Extensive experimental evidence has since demonstrated that cell division cycle protein 45 (Cdc45) is required throughout the process of DNA replication: it is essential for establishment of an initiation complex at DNA origins, and for chromosome unwinding and DNA synthesis at replication forks. More recently, Cdc45 was shown to be an integral component of the Cdc45-MCM-GINS (CMG) assembly responsible for DNA unwinding in the replisome. Recruitment of Cdc45 to the MCM2-7 heterohexamer is a key step in the highly regulated process that leads to the activation of helicase activity. Evidence concerning structure and function of Cdc45 remained elusive, until recent reports identified it as a remote orthologue of bacterial RecJ333435, a 5′-to-3′ single-stranded (ss) DNA exonuclease with multiple roles in DNA repair and a member of the DHH phosphoesterase superfamily.

The X-ray crystal structure of human Cdc45 was solved at 2.1 Å using the anomalous signal of crystals derivatized with the mercury compound thimerosal. A construct with an 11-residue excision (lacking amino acids S154 to I164) crystallized readily and was used for high-resolution structure determination. Crystallographic analysis reveals that human Cdc45 adopts a compact, disk-like shape, resulting from folding of the polypeptide chain into a closed arc, from its N- to the C-terminus. The only deviation from a globular fold is represented by a large helical insertion in the DHH domain, spanning amino acids L118 to S197, which projects away from the folded core of Cdc45 (discussed in detail later); the insertion consists of the low complexity, acidic region, which is almost entirely disordered, followed by the seven-turn helix α6 pointing away from the Cdc45 fold. Our crystallographic analysis shows that Cdc45 bears a remarkable three-dimensional similarity to the RecJ exonuclease, which reveals their homology despite very little sequence identity. The fold consists of an N-terminal DHH domain connected by a three-helix motif (α15 to α17) to a C-terminal DHH-Associated 1 (DHHA1) domain. Superposition with RecJ confirms the identification of Cdc45 residues that occupy equivalent positions to active-site residues in motifs I–IV of RecJ; the structure shows that three out of the four active-site motifs of Cdc45 contain inactivating mutations, providing a structural basis for its known lack of nuclease activity. The structure shows that the DHHA1 loop reaches down across the groove that separates it from the DHH domain and inserts F542 in a hydrophobic pocket on the DHH domain surface, lined by residues A24, G54, W55 and C77 and with V52, L58 as its base. As a result of these interactions, the DHHA1 domain latches onto the DHH domain, causing the steric occlusion of the inter-domain groove, which represents the ssDNA-binding site in RecJ. At its core lies a three-stranded antiparallel β-sheet (β6-8) sandwiched between a long helix (α9) and a helical bundle (α10-14).

> MFVSDFRKEFYEVVQSQRVLLFVASDVDALCACKILQALFQCDHVQYTLVPVSGWQELETAFLEHKEQFHYFILINCGANVDLLDILQPDEDTIFFVCDTHRPVNVVNVYNDTQIKLLIKQDDDLEVPAYEDIFRDEEEDEEHSGNDSDGSEPVEQTMRRRQRREWEARRRDILFDYEQYEYHGTSSAMVMFELAWMLSKDLNDMLWWAIVGLTDQWVQDKITQMKYVTDVGVLQRHVSRHNHRNEDEENTLSVDCTRISFEYDLRLVLYQHWSLHDSLCNTSYTAARFKLWSVHGQKRLQEFLADMGLPLKQVKQKFQAMDISLKENLREMIEESANKFGMKDMRVQTFSIHFGFKHKFLASDVVFATMSLMESPEKDGSGTDHFIQALDSLSRSNLDKLYHGLELAKKQLRATQQTIASCLCTNLVISQGPFLYCSLMEGTPDVMLFSRPASLSLLSKHLLKSFVCSTKNRRCKLLPLVMAAPLSMEHGTVTVVGIPPETDSSDRKNFFGRAFEKAAESTSSRMLHNHFDLSVIELKAEDRSKFLDALISLLS2-(4-methoxyphenyl)sulfanyl-~{N}-(2-methyl-5,6-dihydro-4~{H}-cyclopenta[c]pyrazol-3-yl)ethanamide | C16 H19 N3 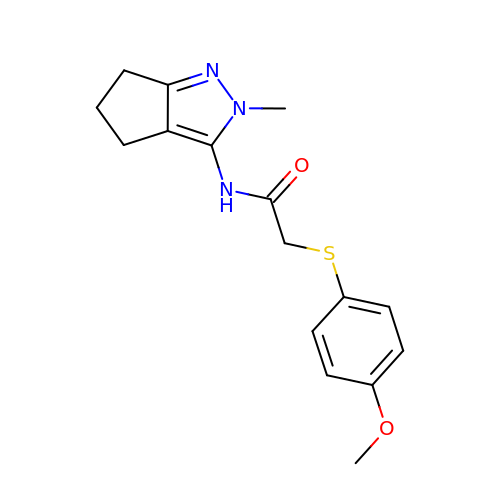O2 S | HLIFAMDWHQBTKJ-UHFFFAOYSA-N> GGAAUCUCGCCCGAUGUUCGCAUCGGGAUUUGCAGGUCCAUGGAUUACACCAUGCAACGCAGACCUGUAGAUGCCACGCUAGCCGUGGUGAGGGUCGGGUCCAGAUGUCAUUCGACUUUAACGCGCCUAAGCGUUGAAGGCGUGUUAGAGCAGAUAGUUCGCUAUCUGGGGAGCCUGUUCGCAGGCUCAGGAGCCUUCGGGCUCCUAGCGCUAUUACCCCGGACACCACCGGGCAGACAAGUAAUGGUGCUCCUCGAAUGACUUCUGUUGAGUAGAGUGUGGGCUCCGCGGCUAGUGUGCACCUUAGCGGUGAAUGUCUGACACCGUUAAGGUGGUUACUCUUCGGAGUAACGCCGAGAUUCC

Here, we use the RNA origami method to prototype an RNA robotic device, named the “Traptamer,” that mechanically traps the fluorescent aptamer, iSpinach. The Traptamer is shown to sense two RNA key strands, acts as a Boolean AND gate, and reversibly controls the fluorescence of the iSpinach aptamer. To construct the Traptamer, we positioned the iSpinach aptamer in the middle helix of a three-helix RNA origami tile, with the outer helices intentionally kept short to force the iSpinach aptamer out of plane and into a deactivated conformation. To enable the trap to open, we integrated branched kissing loops (bKL) into the top and bottom helices.

Last, we use cryo–electron microscopy (cryo-EM) to determine the structure of the closed form of the Traptamer at 5.45-Å resolution, revealing details of the mechanical distortion of the iSpinach motif. To gain a better understanding of the trapped conformation of the iSpinach aptamer, we used cryo-EM to analyze the cotranscriptionally assembled conformation of 14-14 with and without keys. By flexibly fitting the native iSpinach model into our density map, we obtained a model of the deformed state and its effects on the fluorophore binding pocket. In the native state of iSpinach, the fluorophore binding pocket is located between the G4 and an A-U base pair. The cryo-EM model shows that the bending occurs right at the binding pocket, where the A45-U22 base pair occupies the space of the fluorophore. This bending disrupts the triplex lid formed by the A45-U22 base pair and the bulged U42, while the G4s remain generally preserved. The hinge-like deformation provides an explanation for the mechanical deactivation of the iSpinach aptamer inflicted by the forces of bKL formation in the origami frame. Since the G4 of the iSpinach motif is very stable, the deformation occurs at the ligand binding site, leading to the ejection of DFHBI-1T and bending at the empty binding site. Structural investigation of the 14-14 Traptamer using cryo-EM revealed a bending of the iSpinach aptamer caused by the tension induced on the middle helix due to the formation of the bKLs. Thus, 14-14 exhibited cooperative behavior, acting similar to an AND gate, indicating that both bKL A and B were formed and independently inhibited the active form of iSpinach.>[2x]GHMTGPTDATAPARCRVCGDTVDEFLDLGRQPLSDRFLTPADTDGEFFYRLAVGRCHACGMVQLTEEVPRHLMFHEEYPYHSSGSSVMREHFAKVAQRLLATELTGADPFVVEIGCNDGIMLRAVHEAGVRHLGFEPSAGVAEVARSRGVRVRTEFFEKATATAVRESEGPADVIYAANTMCH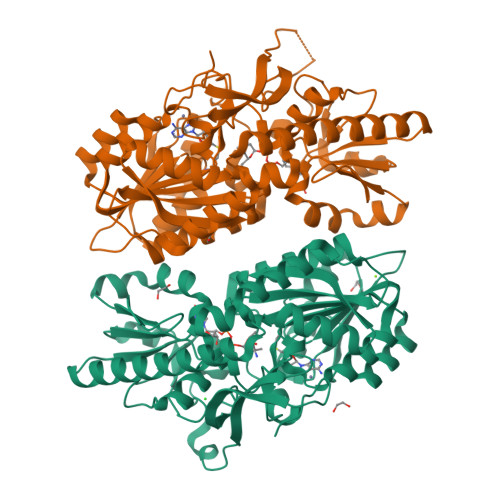IPYLESVFQGADALLGPDGVVVFEDPYLGDIVAKTSFDQIYDEHFYLFSAGSVAAMAERFGFELVDVERLPVHGGEVRYTLARRGARTPTEAVGRLLAEEREQGLDDLATLRTFAANVHTVRDELVALLTRLRAEGHRVVGYGATAKSATVTNFCGIGPDLVSFVCDTTPGKQHRLTPGKHLPVRPAEAFADPYPDYALLFAWNHADEIMAKEQEFRQAGGRWILYVPEVRVL>[2x]GPHMETETSFFDLYDVDLKDKRSVIGKGAFSTVHRCVNKRTGEVCAVKVIALKSLRSSEINKIKREIGICSSLQHEHIVSMRRAFRDESHFYLVFEYVSGGELFDEIVTRKFYNEKDASACMHQILSALQHCHSKNIIHRDLKPENLLLASKDPNAPVKITDFGLAVIMEQGPTYFGFAGTPGYLSPEVIRRVPYDTAVDVWACGVILYILLVGYPPFWEEDHQKLYAQIKNCQYDFPSPEWDSVTTAAKELIKAMLEPNPKRRPTVQELLQHPWIARRDVPGSVHRQATLEELKKFNARRKLKGGVNAVIGVSKMMRTMQEATRALTLSAKSAAALEHHHHHH

Ca2+/calmodulin-dependent protein kinase II (CaMKII) is a Ser/Thr kinase that is particularly important in neuronal signaling and cardiac function. CaMKII has a unique architecture, in which the catalytic domains are linked flexibly to a hub domain, also called the association domain, which forms a dodecameric or tetradecameric assembly (see Figure 1A for a description of the domains of CaMKII). We reported recently that the activation of CaMKII-α by ATP and Ca2+/CaM triggers the exchange of activated subunits between different holoenzyme assemblies. Our data are consistent with the idea that the CaM-binding element induces the hub to transition from a closed-ring form to a ring-opened lock-washer configuration, which can release or capture dimer units.

The S. rosetta kinase domain, including the autoinhibitory segment, and the hub are 52% and 41% identical in sequence to the corresponding domains of human CaMKII-α. Although S. rosetta CaMKII contains a residue that is equivalent to Thr 286, it lacks the two inhibitory phosphorylation sites within the CaM-binding element of the autoinhibitory segment (Thr 305 and Thr 306), as well as sites of regulatory glycosylation, nitrosylation and oxidation. We expressed, purified, and crystallized the kinase and hub domains of S. rosetta CaMKII separately.XIAP (X-linked inhibitor of apoptosis) directly inhibits the upstream caspase-9 and the downstream caspase-3 and caspase-7, and therefore controls critical apoptotic checkpoints. The XIAP protein consists of several domains, including three zinc-containing BIR (baculovirus IAP repeat) domains (BIR1, BIR2 and BIR3) and a C-terminal RING domain. The linker region blocks the active sites of these caspases, while the N-terminal regions of the partially processed caspase-3 and caspase-7 bind the BIR2 domain in a peptide-binding groove that accommodates the four N-­terminal residues. As has been reported previously for other BIR domains, the overall architecture of the BIR2 domain is a three-stranded antiparallel β-sheet surrounded by five α-helices, with a structurally important zinc residue coordinated by Cys200, Cys203, His220 and Cys227.

Therefore, the structures of XIAP BIR2 with five different peptides soaked in and bound to the Smac binding groove were also solved: ATAA, AVPI, SVPI, AIAV and AMRV. P2 makes standard backbone-to-backbone hydrogen-bond interactions with BIR2, and the side chain points towards solvent. The only interactions are hydrophobic ones with the side chains of Asn209 and Lys208, perhaps leading to the weak preference of BIR2 for hydrophobic residues at P2 (see the AMRV structure), but explaining the general lack of strong preferences for this residue. The methionine at P2 shows how the side chains of Asn209 and Lys208 can flank and provide a hydrophobic environment for a longer P2 side chain. Owing to the large arginine at P3, there must be a compensatory shift in the peptide backbone in order to allow the side chain room to fit, since the Cα—Cβ bond of the arginine lies flat against the protein (as was noted for ATAA). While the P4 valine only needs a shallow pocket, the P3 shift is large enough that the P4 NH to Leu207 backbone interaction is lost.

>[2x]GTIYPRNPAMYSEEARLKSFQNWPDYAHLTPRELASAGLYYTGIGDQVQCFACGGKLKNWEPGDRAWSEHRRHFPNCFFVLGRNLN;> AMRV>GSAKDLSATSTTSSTTAFSATTAGNAIAGKYTISVTHLAQAQTLTTRTTRDDTKTAIATSDSKLTIQQGGDKDPITIDISAANSSLSGIRDAINNAKAGVSASIINVGNGEYRLSVTSNDTGLDNAMTLSVSGDDALQSFMGYDASASSNGMEVSVAAQNAQLTVNNVAIENSSNTISDALENITLNLNDVTTGNQ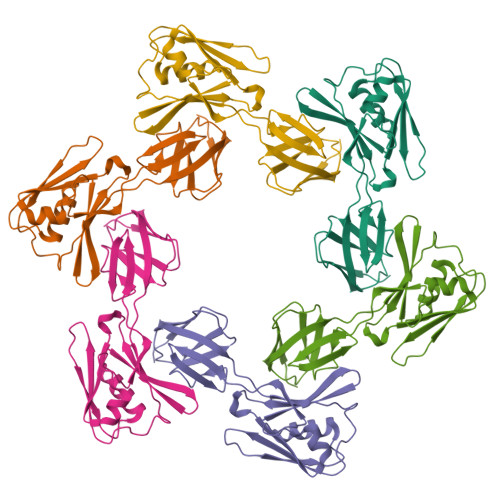TLTITQD[2x]>[2x]MAPTFQTALFFTIISLSFAAPNAKQVRWCAISDLEQKKCNDLVGSCNVPDITLVCVLRSSTEDCMTAIKDGQADAMFLDSGEVYEASKDPYNLKPIIAEPYSSNRDLQKCLKERQQALAKKMIGHYIPQCDEKGNYQPQQCHGSTGHCWCVNAMGEKISGTNTPPGQTRATCERHELPKCLKERQVALGGDEKVLGRFVPQCDEKGNYEPQQFHGSTGYSWCVNAIGEEIAGTKTPPGKIPATCQKHDLVTTCHYAVAMVKKSSAFQFNQLKGKRSCHSGVSKTDGWKALVTVLVEKKLLSWDGPAKESIQRAMSKFFSVSCIPGATQTNLCKQCKGEEGKNCKNSHDEPYYG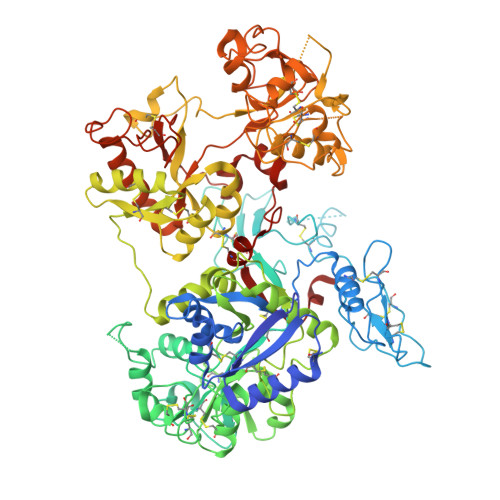NYGAFRCLKEDMGDVAFLRSTALSDEHSEVYELLCPDNTRKPLNKYKECNLGTVPAGTVVTRKISDKTEDINNFLMEAQKRQCKLFSSAHGKDLMFDDSTLQLALLSSEVDAFLYLGVKLFHAMKALTGDAHLPSKNKVRWCTINKLEKMKCDDWSAVSGGAIACTEASCPKGCVKQILKGEADAVKLEVQYMYEALMCGLLPAVEEYHNKDDFGPCKTPGSPYTDFGTLRAVALVKKSNKDINWNNIKGKKSCHTGVGDIAGWVIPVSLIRRQNDNSDIDSFFGESCAPGSDTKSNLCKLCIGDPKNSAANTKCSLSDKEAYYGNQGAFRCLVEKGDVAFVPHTVVFENTDGKNPAVWAKNLKSEDFELLCLDGSRAPVSNYKSCKLSGIPPPAIVTREESISDVVRIVANQQSLYGRKGFEKDMFQLFSSNKGNNLLFNDNTQCLITFDRQPKDIMEDYFGKPYYTTVYGASRSAMSSELISACTIKHCSNSLEVLFQ> DAIDALSSDF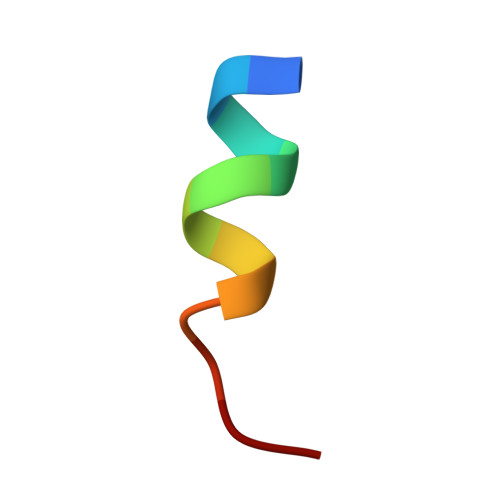TS1-{(2S,5R)-2-methyl-5-[(7H-pyrrolo[2,3-d]pyrimidin-4-yl)amino]piperidin-1-yl}propan-1-one | C15 H21 N5 O | 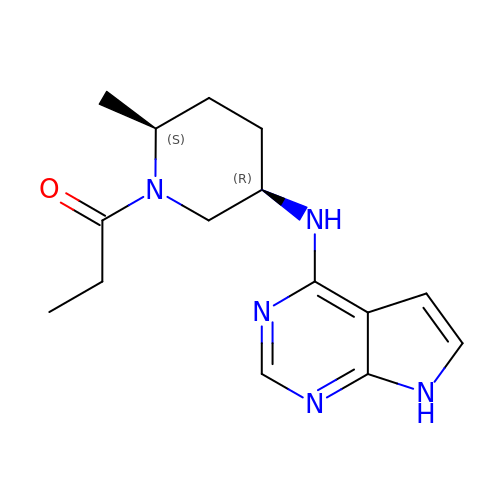VCTGEVNTYUYDAZ-WDEREUQCSA-N>[2x]MNPLDLIAKRAYPYETEKRDKTYLALNENPFPFPEDLVDEVFRRLNSDALRIYYDSPDEELIEKILSYLDTDFLSKNNVSVGNGADEIIYVMMLMFDRSVFFPPTYSCYRIFAKAVGAKFLEVPLTKDLRIPEVNVGEGDVVFIPNPNNPTGHVFE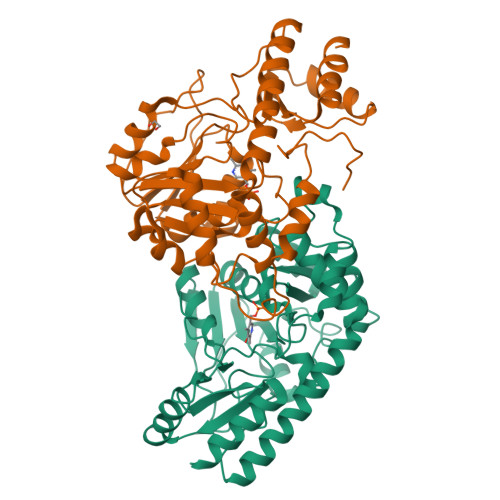REEIERILKTGAFVALDEAYYEFHGESYVDFLKKYENLAVIRTFSKAFSLAAQRVGYVVASEKFIDAYNRVRLPFNVSYVSQMFAKVALDHREIFEERTKFIVEERERMKSALREMGYRITDSRGNFVFVFMEKEEKERLLEHLRTKNVAVRSFREGVRITIGKREENDMILRELEVFK>[2x]SNAMKSIILIVLDGLGDRPGSDLQNRTPLQAAFRPNLNWLASHGINGIMHPISPGIRCGSDTSHMSLLGYDPKVYYPGRGPFEALGLGMDIRPGDLAFRANFATNRDGVIVDRRAGRENKGNEELADAISLDMGEYSFRVKSGVEHRAALVVSGPDLSDMIGDSDPHREGLPPEKIRPTDPSGDRTAEVMNAYLEEARRIL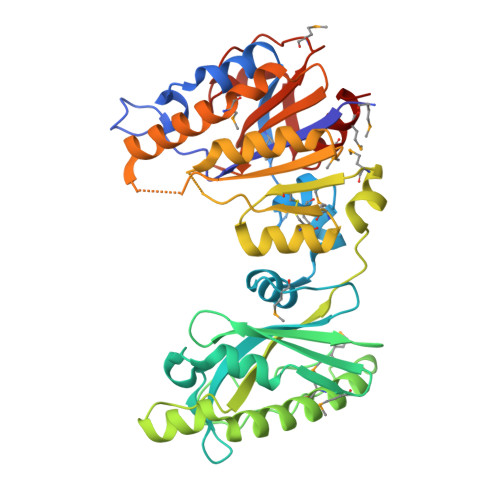SDHRVNKERVKNGRLPGNELLVRSAGKVPAIPSFTEKNRMKGACVVGSPWLKGLCRLLRMDVFDVPGATGTVGSNYRGKIEKAVDLTSSHDFVLVNIKATDVAGHDGNYPLKRDVIEDIDRAMEPLKSIGDHAVICVTGDHSTPCSFKDHSGDPVPIVFYTDGVMNDGVHLFDELSSASGSLRITSYNVMDILMQLAG> MEEPEEPADSGQSLVPVYIYSPEYVSMCDS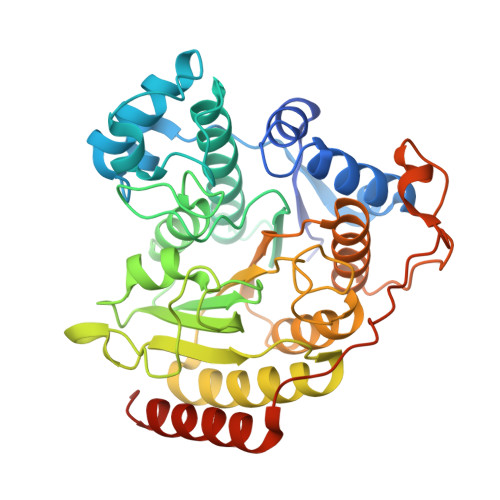LAKIPKRASMVHSLIEAYALHKQMRIVKPKVASMEEMATFHTDAYLQHLQKVSQEGDDDHPDSIEYGLGYDCPATEGIFDYAAAIGGATITAAQCLIDGMCKVAINWSGGWHAAKKDEASGFCYLNDAVLGILRLRRKFERILYVDLDLHHGDGVEDAFSFTSKVMTVSLHKFSPGFFPGTGDVSDVGLGKGRYYSVNVPIQDGIQDEKYYQICESVLKEVYQAFNPKAVVLQLGADTIAGDPMCSFNMTPVGIGKCLKYILQWQLATLILGGGGYNLANTARCWTYLTGVILGKTLSSEIPDHEFFTAYGPDYVLEITPSCRPDRNEPHRIQQILNYIKGNLKHVVIEGRSHHHHHH> XLDLNFKLLEEHLA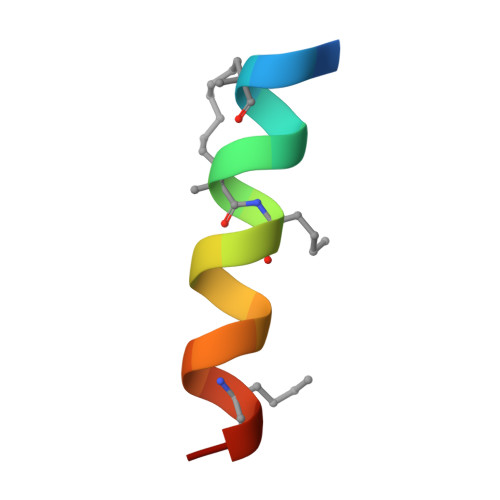LLVEX> GMDRTLTHQPQEYA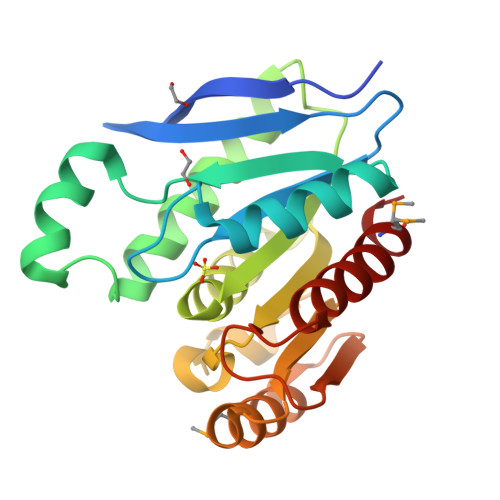VSVSVGEVKLKGNLVIPNGATGIVLFAHGSGSSRYSPRNRYVAEVLQQAGLATLLIDLLTQEEEEIDLRTRHLRFDIGLLASRLVGATDWLTHNPDTQHLKVGYFGASTGGGAALVAAAERPETVQAVVSRGGRPDLAPSALPHVKAPTLLIVGGYDLPVIAMNEDALEQLQTSKRLVIIPRASHLFEEPGALTAVAQLASEWFMHYLR> MIRDIIRMGDKRLLRVAPQVTNLGSAELHALVSDMFETMGAAHGVGLAAPQIAVDLQLMVFGFEASERYPEAPAVPLTALANAQIEPLSDEMENGWEGCLSIPGLRAVIPRYRYIRYRGFAP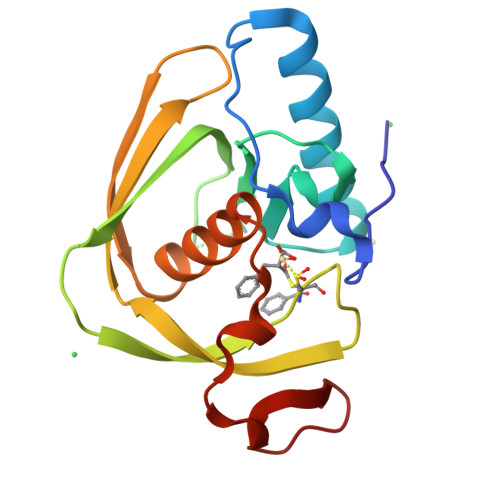DGSPIEREAEGFHARVVQHEYDHLVGRLYPSRIENFDTFGFDDVLSY> MSDGAVQPDGGQPAVRNERATGSGNGSGGGGGGGSGGVGISTGTFNNQTEFKFLENGWVEITANSSRLVHLNMPESENYKRVVVNNMDKTAVKGNMALDDIHVEIVTPWSLVDANAWGVWFNPGDWQLIVNTMSELHLVSFEQEIFNVVLKTVSESATQPPTKVYNNDLTASLMVALDSNNTMPFTPAAMRSETLGFYPWKPTIPTPWRYYFQWDRTLIPSHTGTSGTPTNVYHGTDPDDVQFYTIENSVPVHLLRTGDEFATGTFFFDCKPCRLTHTWQTNRALGLPPFLNSLPQSEGATNFGDIGVQQDKRRGVTQMGNTDYITEATIMRPAEVGYSAPYYSFEASTQGPFKTPIAAGRGGAQTDENQAADGDPRYAFGRQHGQKTTTTGETPERFTYIAHQDTGRYPEGDWIQNINFNLPVTNDNVLLPTDPIGGKTGINYTNIFNTYGPLTALNNVPPVYPNGQIWDKEFDTDLKPRLHINAP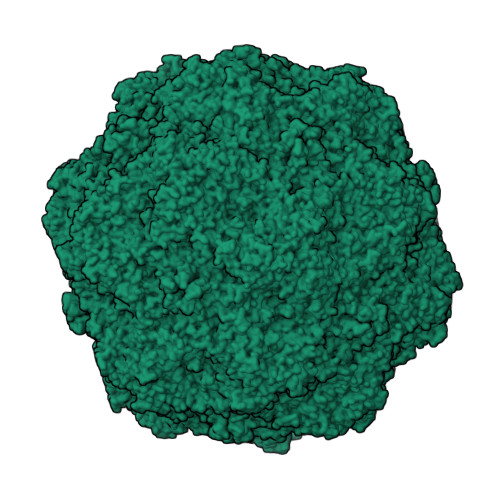FVCQNNCPGQLFVKVAPNLTNQYDPDASANMSRIVTYSDFWWKGKLVFKAKLRASHTWNPIQQMSINVDNQFNYVPNNIGAMKIVYEKSQLAPRKLY4-cyanobenzenesulfonic acid | C7 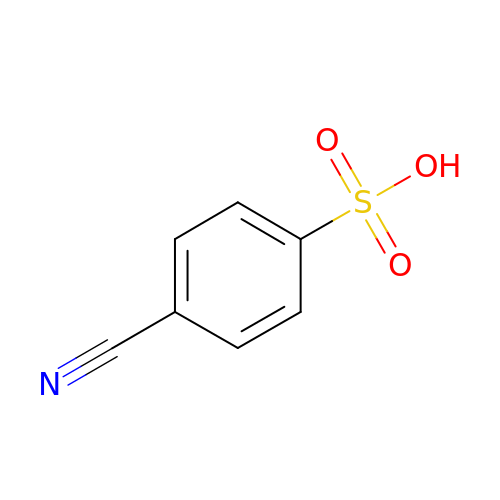H5 N O3 S | SLBRSTXWIBNAOM-UHFFFAOYSA-N[[[3-(2-METHYL-PROPANE-2-SULFONYL)-1-BENZENYL]-2-PROPYL]-CARBONYL-HISTIDYL]-AMINO-[CYCLOHEXYLMETHYL]-[2-HYDROXY-4-ISOPROPYL]-PENTAN-5-OIC 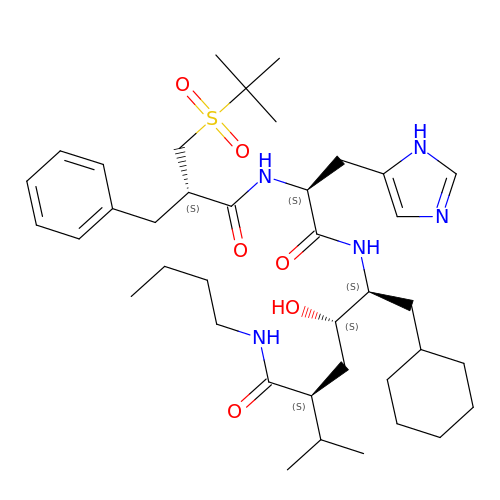ACID BUTYLAMIDE | C39 H63 N5 O6 S | GGKXIITZBSPCQP-IZIWAXSGSA-N> XHGLDDAQYLQQKAHNKRISEFRSSSNSGINVTVVLKYTNGVVQVYNWQGTEVIAGSLNRQLMKFPNYMNPDKHGRIEWPGEGVEHQHGLIRSNGGNGSYDIGAGDPYAMQFIVQGSVDWNATRLRFFGPDGSRWMPDDQGGASVRAGLLNAAEDIINSKMQPLYFCDRMAGKSYYVRFDDKYAPRFPTIGFEVYRYRVGATN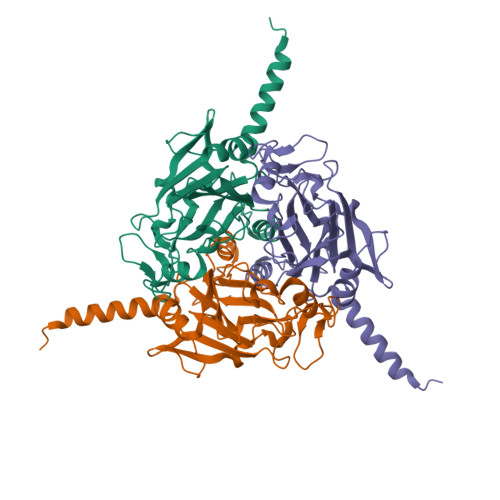EMGGESARTAVASLISFPTFSTAYVNEKVAVENFFQPRELVYQNSYGYTV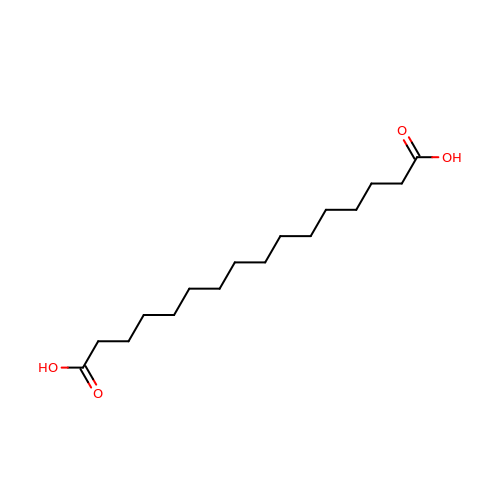hexadecanedioic acid | C16 H30 O4 | QQHJDPROMQRDLA-UHFFFAOYSA-N>MGSSHHHHHHSSGRENLYFQGHMSRNLLAIVHPILRNLMEESGETVNMAVLDQSDHEAIIIDQVQCTHLMRMSAPIGGKLPMHASGAGKAFLAQLSEEQVTKLLHRKGLHAYTHATLVSPVHLKEDLAQTRKRGYSFDDEEHALG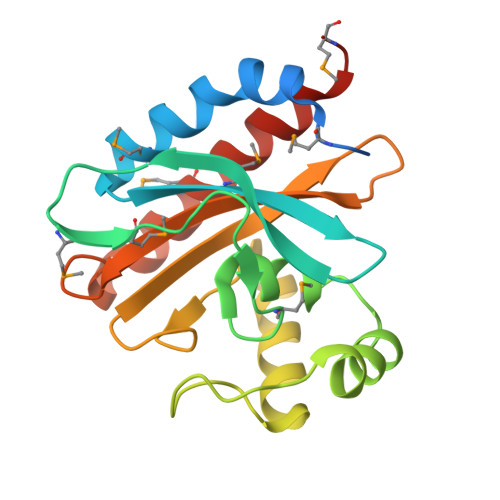LRCLAACIFDEHREPFAAISISGPISRITDDRVTEFGAMVIKAAKEVTLAYGGMRGS[4x]>MDPKISEMHPALRLVDPQIQLAVTRMENAVGRDQNNVGPKVYPIILRLGSPLSLNMARKTLNSLEDKAF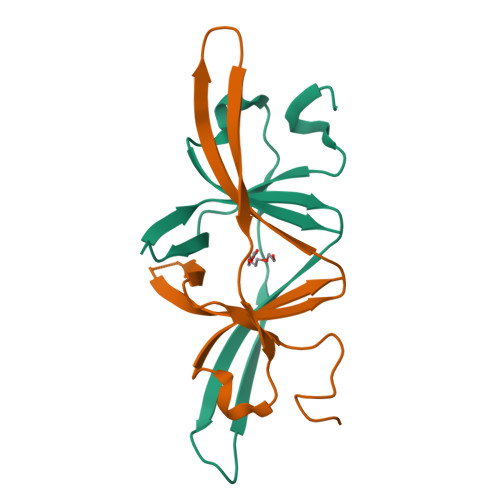QLTPIAVQMTKLATTEELPDEFVVVTVK[2x]>MKTVVFAYHDMGCLGIEALLAAGYEISAIFTHTDNPGEKAFYGSVARLAAERGIPVYAPDNVNHPLWVERIAQLSPDVIFSFYYRHLIYDEILQLAPAGAFNLHGSLLPKYRGRAPLNWVLVNGETETGVTLHRMVKRADAGAIVAQLRIAIAPDDIAITLHHKLCHAARQLLEQTLPAIKHGNILEIAQRENEATCFGRRTPDDSFLEWHKPASVLHNMVRAVADPWPGAFSYVGNQKFTVWSSRVHPHASKAQPGSVISVAPLLIACGD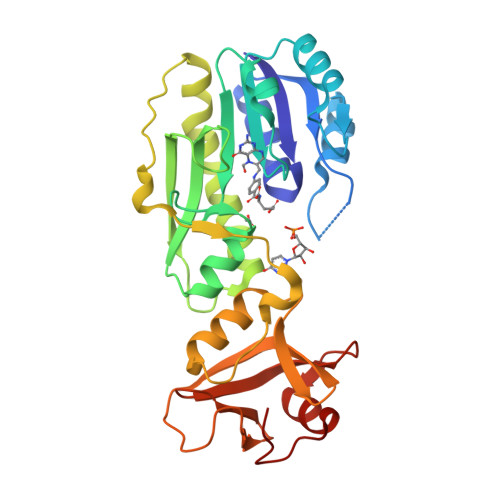GALEIVTGQAGDGITMQGSQLAQTLGLVQGSRLN[2x]> FEGDLKWHHHNITYWIQNYSEDLPRAVIDDAFARAFALWSAVTPLTFTRVYSRDADIVIQFGVAEHGDGYPFDGKDGLLAHAFPPGPGIQGDAHFDDDELWSLGKGVGYSLFLVAAHQFGHALGLDHSSVPEALMYPMYRFTEG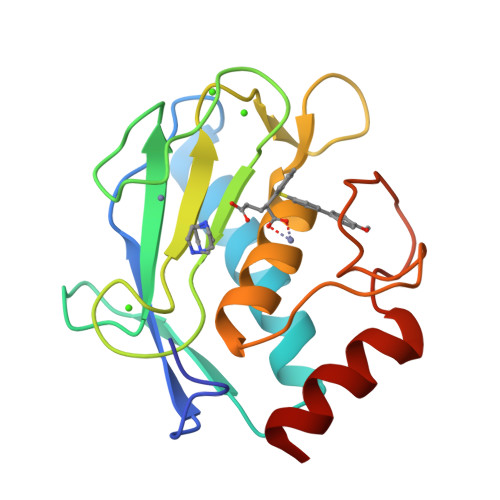PPLHKDDVNGIRHLYG>MAHHHHHHSSGLEVLFQGPNNTIINSLIGGDDSIKRSNVFAVDSQIPTLYMPQYISLSGVMTNDGPDNQAIASFEIRDQYITALNHLVLSLELPEVKGMGRFGYVPYVGYKCINHVSISSCNGVIWEIEGEELYNNCINNTIALKHSGYSSELNDISIGLTPN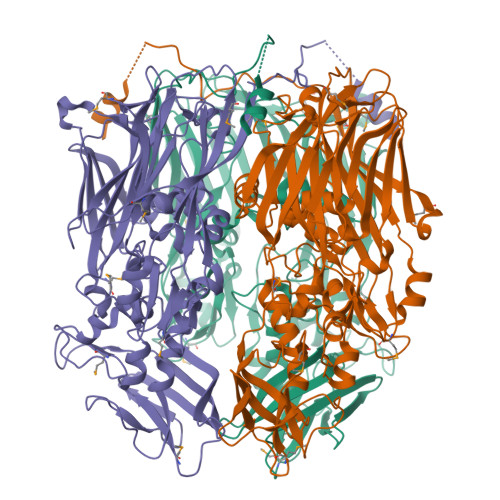DTIKEPSTVYVYIKTPFDVEDTFSSLKLSDSKITVTVTFNPVSDIVIRDSSFDFETFNKEFVYVPELSFIGYMVKNVQIKPSFIEKPRRVIGQINQPTATVTEVHAATSLSVYTKPYYGNTDNKFISYPGYSQDEKDYIDAYVSRLLDDLVIVSDGPPTGYPESAEIVEVPEDGIVSIQDADVYVKIDNVPDNMSVYLHTNLLMFGTRKNSFIYNISKKFSAITGTYSDATKRTIFAHISHSINIIDTSIPVSLWTSQRNVYNGDNRSAESKAKDLFINDPFIKGIDFKNKTDIISRLEVRFGNDVLYSENGPISRIYNELLTKSNNGTRTLTFNFTPKIFFRPTTITANVSRGKDKLSVRVVYSTMGVNHPIYYVQKQLVVVCNDLYKVSYDQGVSITKIMGDNN[3x]(METHYLPYRIDAZINE PIPERIDINE PROPYLOXYPHENYL)ETHYLACETATE 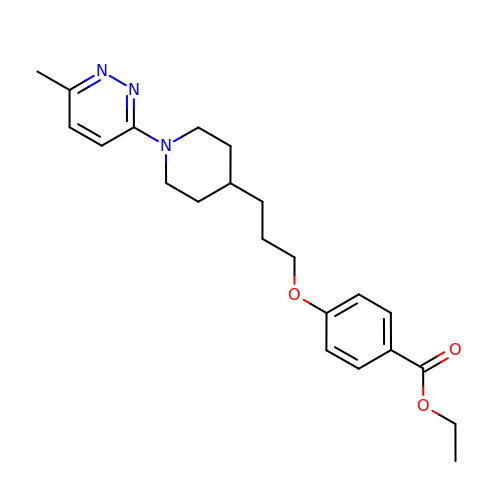| C22 H29 N3 O3 | UEIUDEUUVLYRFV-UHFFFAOYSA-N Ribosome inactivating proteins (RIPs) are enzymes that can inactivate ribosomes. The molecular mechanism of inhibitory effect on protein synthesis has been shown that RIPs act as a RNA N-glycosidase hydrolyzing the C-N glycosidic bond of the adenosine residue at position 4324 in rat 28S rRNA. Some are type II RIPs consisting of two types of polypeptide subunits, A chain of homologous and functionally similar to type I RIPs and B chain with a galactose-specific lectin domain that binds to cell surfaces, such as ricin abrin and abrus agglutinin (AAG). Abrins are potent toxic heterodimeric glycoproteins with an LD50 of 20 μg/kg body weight; while AAG is a relatively less toxic heterotetrameric glycoprotein of which the LD50 is 5 mg/kg body weight.

We have successfully solved the structure of 120 kDa heterotetramer agglutinin AB and CD chains, and reduced the R-factor to 20.4% at 2.6 Å resolution data. The AAG AB-chains are very similar to the abrin-a molecule, the structure of which has been described in detail. A conserved disulfide bond between Cys246 of A (or C)-chain and Cys8 of B (or D)-chain holds the two chains tightly as shown in figure 1. Two NAGs are found in B-chain, but only one presents in D chain. An AAG molecule is a hetero-tetramer contains two subunits, ABA'B' (or CDC'D'), stabilized by mainly hydrophilic and little hydrophobic forces. 22 hydrogen bonds between A (or C)-chain and symmetry-related A' (or C') were found. The active site is exactly the cleft formed by the intersection of all 3 domains in AAG A (or C)-chain. Five invariant residues (Tyr73, Tyr112, Glu163, Arg166 and Trp197) and five conserved residues (Asn71, Arg123, Gln159, Glu194 and Asn195) are located in the active site cleft. Docking study revealed that due to Pro199, agglutinin is unable to form a critical hydrogen bond with G4323 of 28SRNA, which is found in the docking result of abrin-a. This may explain the lower toxicity of agglutinin than abrin-a, despite of similarity in secondary structure and the activity cleft of two RIPs.

>[2x]QDPIKFTTGSATPASYNQFIDALRERLTGGLIYGIPVLRDPSTVEKPNQYVTVELSYSDTVSIQLGIDLTNAYVVAYRAGSESFFFRNAPASASTYLFTGTQQYSLPFDGNYDDLEKWAHQSRQRISLGLEALRQGIKFLRSGASDDEEIARTLIVIIQMVAEAARFRYVSKLVVISLSNRAAFQPDPSMLSLENTWEPLSRAVQHTVQDTFPQNVTLINVRQERVVVSSLSHPSVSALALMLFVCNPLNATQSPLLI;>VVEQSKICSSHYEPTVRIGGRDGLCVDVSDNAYNNGNPIILWKCKDQLEVNQLWTLKSDKTIRSKGKCLTTYGYAPGNYVMIYDCSSAVAEATYWDIWDNGTIINPKSGLVLSAESSSMGGTLTVQKNDYRMRQGWRTGNDTSPFVTSIAGFFKLCMEAHGNSMWLDVCDITKEEQQWAVYPDGSIRPVQNTNNCLTCEEHKQGATIVMMGCSNAWASQRWVFKSDGTIYNLYDDMVMDVKSSDPSLKQIILWPYTGNANQMWATLF[2x]> MANEELTESQQQEDPSQQLPNADEEKGSDSDSNSDSDASSQSSGDDFYISESEN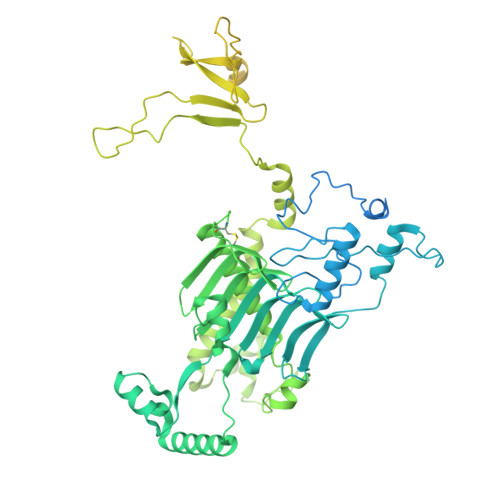EAEGDNTIFNYVRPSDIPPDPNANPETNIRRFNRVLDGKRVKRMQEEEEDKYTFYEDLFDFPRDPERWKEQDLREIWADGPLEMTKPGWDPAWADEDDWDVVNDEIQEGRDPGIQPFYVPYRKPYPAIPDNHYDIENAKGVVEELDRIEEFLQWVSYIFPDGSSYEGTVWDDLAQGKGVYIAENGLVRYEGEWLQNDMEGHGVIDVDIPDIEPIPGSKLEAKMRAEGRIIKRDYMTPEDRKWLEMDVEDSVALTDGNFQVPFYENEEWVTQFGEKPEKGRYRYAGQWKHSRMHGCGVYEVNERILYGRFYFGELLEEEHGCTVDICALHSGLAEVAAAKARMFVNKPDGMIREERGPYGDPQHPYFYEEDDVWMAPGFINQFYEVPEYWETYVGEVDQEREMWLNSFYKAPLRLPMPAELEHWWENVEVTPEFVLLNKEPEPDPNDPSKLVQKEDPVILHTPTGRIINYVEDEKHGIRLFWQPPLEEGEEVDPSKVEFLPLGFDEFYGKEVVVKKEHPIKSFVLGIEKSVKPMLDGLEKWTEEKKKAYEERKEMIQQELELVEAEICLEEAIEDMDEELKKKEQEEEKKTEMGLTEEDEDVLVPVYKEEKVVTAKEKIQENKQEEKYKDDDDEDDDDGDDDDDDDDDDDLGPSSFGSADKGRRNSPFSSSSLSFASCTLFPAVQSRLESSFLAWKQHRAEPSKVNTGIIKGADTASASIHFPPLSSNNARLKMGKVANRGCVQRSYGSSRSQSQLMSLSRLLSCNASSSSSPPDSSSSEYLKDSGLWETPVGDMSVVLSLQIQTKCSDLFAETPAVS> MEDTAVETKAKPEKYGSFSEDSLYSLLVAELAGQRNRFDIALSNYVVQAQKTRDPGVSERAFRIAEYLGADQEALDTSLLWARSAPDNLDAQRAAAIQLARAGRYEESMVYMEKVLNGQGDTHFDFLALSAAETDPDTRAGLLQSFDHLLKKYPNNGQLLFGKALLLQQDGRPDEALTLLEDNSASRHEVAPLLLRSRLLQSMKRSDEALPLLKAGIKEHPDDKRVRLAYARLLVEQNRLDDAKAEFAGLVQQFPDDDDLRFSLALVCLEAQAWDEARIYLEELVERDSHVDAAHFNLGRLAEEQKDTARALDEYAQVGPGNDFLPAQLRQTDVLLKAGRVDEAAQRLDKARSEQPDYAIQLYLIEAEALSNNDQQEKAWQAIQEGLKQYPEDLNLLYTRSMLAEKRNDLAQMEKDLRFV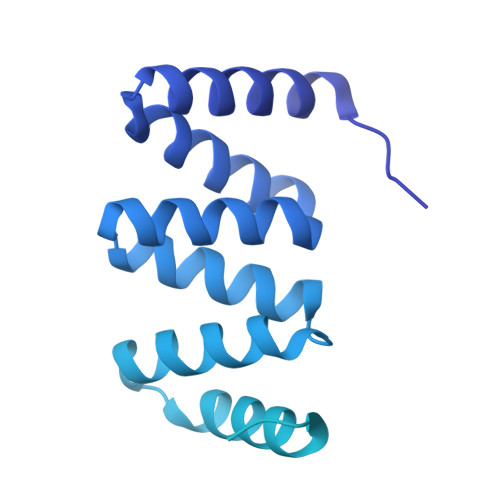IAREPDNAMALNALGYTLADRTTRYGEARELILKAHKLNPDDPAILDSMGWINYRQGKLADAERYLRQALQRYPDHEVAAHLGEVLWAQGRQGDARAIWREYLDKQPDSDVLRRTIKRLTGAETP> AQVDLLNVKGEKVGTLEISDFVFNIDPNYDVMWRYVDMQLSNRRAGTASTKTRGEVSGGGRKPWPQKHTGRARHGSIRSPIWRHGGVVHGPKPRDWSKKLNKKMKKLALRSALSVKYRENKLLVLDDLKLERPKTKSLKEILQNLQLSDKKTLIVLPWKEEGYM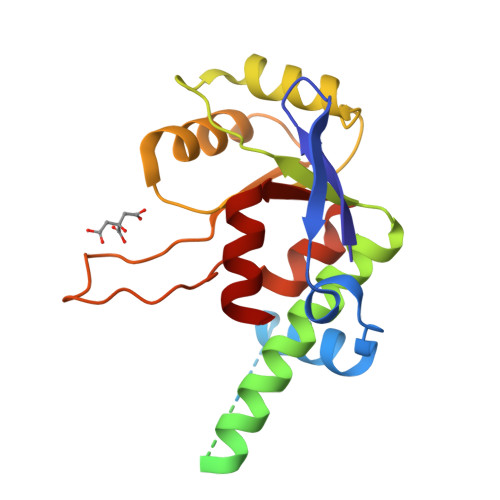NVKLSGRNLPDVKVIIADNPNNSKNGEKAVRIDGLNVFDMLKYDYLVLTRDMVSKIEEVLG>[2x]SMLQSNEYFSGKVKSIGFTSSSTGRASVGVMAEGEYTFGTAEPEEMT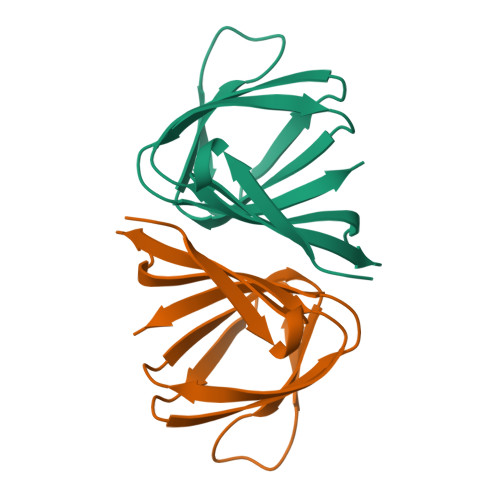VVSGALKVLLPGTVEWKVYTAGEVFNVPGHSEFHLQVAEPASYLCRYL Among the few cytoplasmic enzymes isolated from S. ruber, the tetrameric malate dehydrogenase (MalDH) remains the most extensively characterized, at the biochemical and structural level. Sr MalDH shares more than 72% of sequence similarity with its non-halophilic counterpart Ca MalDH. In our follow-up crystallographic study on Sr MalDH; we determined the direct effect on solvent organization due to its acidic surface, by using a comparison with a non-halophilic counterpart.

For this purpose, we solved de novo the crystal structure of the non-halophilic Chloroflexus aurantiacus (Ca) MalDH at 1.7 Å resolution. It allowed the determination of a hydration shell consisting in 945 water molecules, which cluster themselves in large networks of structured water through pentameric/hexameric polygons. The asymmetric unit contains a dimer, the physiological tetramer being generated by the crystal symmetry operators of the P3121 space group. Moreover, the mobile loop (residues 83–89, following the linear numbering of 4BGT) covering the catalytic site, as well as the residues of the N- and C- termini have been modeled in each monomer of this new Ca MalDH structure. The most interesting feature of the water molecules in Ca MalDH structure is that 28% of them are organized in polygons (pentagons or hexagons), which can form extended clusters. These polygons are only observed at the surface of apolar residues. Around apolar surfaces of the non-halophilic MalDH, water molecules cannot form direct hydrogen bonds with the protein, and thus organize themselves as polygons with their nearest stable water neighbors. As mentioned, large networks of connected water polygons are present in Ca MalDH. In the same protein region, no water polygon is observed in Sr MalDH, which possesses four extra negative charges compared to Ca MalDH, due to substitutions at positions 199, 203, 283, and 285.

>[2x]MRKKISIIGAGFVGSTTAHWLAAKELGDIVLLDIVEGVPQGKALDLYEASPIEGFDVRVTGTNNYADTANSDVIVVTSGAPRKPGMSREDLIKVNADITRACISQAAPLSPNAVIIMVNNPLDAMTYLAAEVSGFPKERVIGQAGVLDAARYRTFIAMEAGVSVEDVQAMLMGGHGDEMVPLPRFSTISGIPVSEFIAPDRLAQIVERTRKGGGEIVNLLKTGSAYYAPAAATAQMVEAVLKDKKRVMPVAAYLTGQYGLNDIYFGVPVILGAGGVEKILELPLNEEEMALLNASAKAVRATLDTLKSL>MDIVAPDRTRIAPEIDRDEALEGDRESDPALASTREWQLEDMPRWQDELTVRGLVAALLIGFIYTVIVMKIALTTGLVPTLNVSAALLSFLALRGWTRLLERFGVVSRPFTRQENTIVQTCGVACYTIAFAGGFGSTLLGLNKKTYELAGDSPGNVPGSWKEPGIGWMTGFLLACSFGGLLTLIPLRQVLVVDYKLVYPSGTATAILINGFHTDQGDKNSRKQIRGFLKYFGGSFLWSFFQWFYTGGDACGFVQFPTFGLKAWKQTFYFDFSMTYVGAGMICPHIVNISTLLGAIISWGIMWPLISKNKGDWYPAKVPESSMKSLYGYKAFICIALIMGDGMYHFIKIVGITAMSMYRQFSHKQVNNKAKNADDTVSLEELHRQEIFKRGHIPSWMAYAGYALFSVLAVVTIPVMFKQVKWYYVVIAYVVAPMLGFANSYGTGLTDINMGYNYGKIALFVFAGWAGKENGVIAGLVAGTLVKQLVLISADLMQDFKTSYLTQ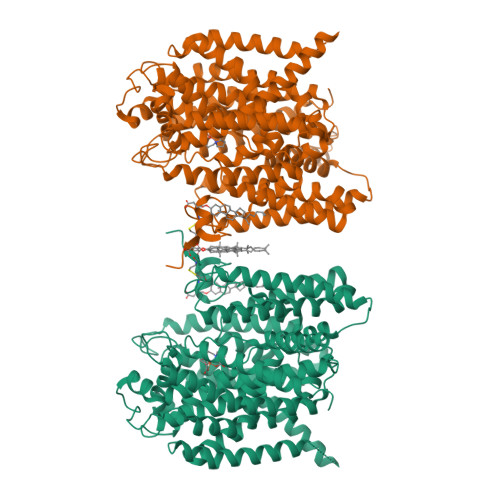TSPKSMMIAQVVGTAMGCIVSPLTFMLFYKAFDIGNPDGTWKAPYALIYRNMAILGVEGFSVLPKYCIVISGGFFAFAAILSITRDVMPHKYAKYVPLPMAMAVPFLVGGSFAIDMCLGSLIVFAWTKINKKEAGFMVPAVASALICGDGIWTFPASILALAKIKPPICMKFLPAATSAAHHHHHHHH[2x]1-(4-chloranyl-2,3-dihydroindol-1-yl)ethanone | C10 H10 Cl N O | 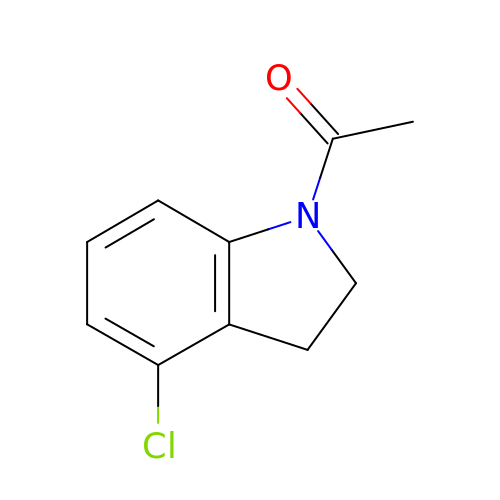PRQBPDDBVHPKIP-UHFFFAOYSA-N> NDKLVELSKSDDNWVMPGKNYDSNNFSDLKQINKGNVKQLRPAWTFSTGLLNGHEGAPLVVDGKMYIHTSFPNNTFALGLDDPGTILWQDKPKQNPAARAVACCDLVNRGLAYWPGDGKTPALILKTQLDGNVAALNAETGETVWKVENSDIKVGSTLTIAPYVVKDKVIIGSSGAELGVRGYLTAYDVKTGEQVWRAYATGPDKDLLLASDFNIKNPHYGQKGLGTGTWEGDAWKIGGGTNWGWYAYDPGTNLIYFGTGNPAPWNETM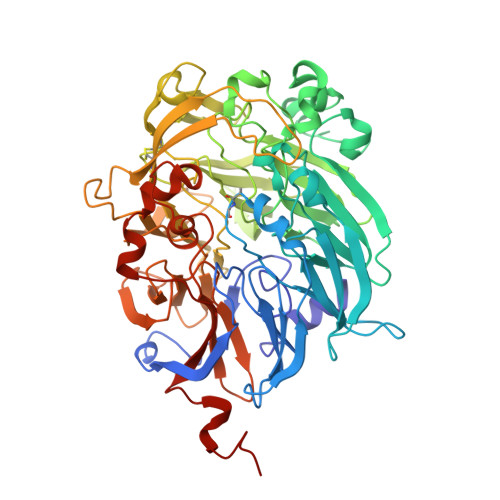RPGDNKWTMTIFGRDADTGEAKFGYQKTPHDEWDYAGVNVMMLSEQKDKDGKARKLLTHPDRNGIVYTLDRTDGALVSANKLDDTVNVFKSVDLKTGQPVRDPEYGTRMDHLAKDICPSAMGYHNQGHDSYDPKRELFFMGINHICMDWEPFMLPYRAGQFFVGATLNMYPGPKGDRQNYEGLGQIKAYNAITGDYKWEKMERFAVWGGTMATAGDLVFYGTLDGYLKARDSDTGDLLWKFKIPSGAIGYPMTYTHKGTQYVAIYYGVGGWPGVGLVFDLADPTAGLGAVGAFKKLANYTQMGGGVVVFSLDGKGPYDDPNVGEWKSAAK> LLQHVKFQSSNFENILTWDSGPEGTPDTVYSIEYKTYGERDWVAKKGCQRIT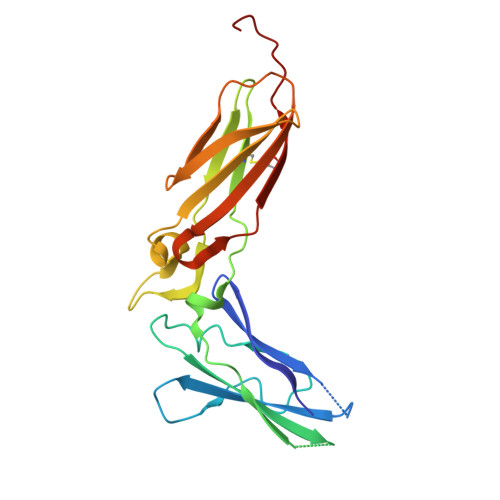RKSCNLTVETGNLTELYYARVTAVSAGGRSATKMTDRFSSLQHTTLKPPDVTCISKVRSIQMIVHPTPTPIRAGDGHRLTLEDIFHDLFYHLELQVNRTYQMHLGGKQREYEFFGLTPDTEFLGTIMICVPTWAKESAPYMCRVKTLPDRTWTG>[2x]GKITLYEDRGFQGRHYECSSDHPNLQPYLSRCNSA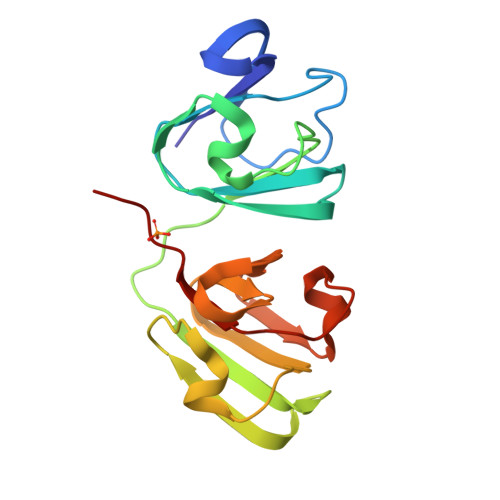RVDSGCRMLYEQPNYSGLQYFLRRGDYADHQQWMGLSDSVRSCRLIPHSGSHRIRLYEREDYRGQMIEFTEDCSCLQDRFRFNEIHSLNVLEGSWVLYELSNYRGRQYLLMPGDYRRYQDWGATNARVGSLRRVIDFS> MAPRNEIEETLVTIWQDVLGIEKIGIKDNFYALGGDSIKAIQVAARLHSYQLKLETKDLLKYPTIDQLVHYIKDSKRRSEQGIVEGEIGLTPIQHWFFEQQFTNMHHWNQSYMLYRPNGFDKEILLRVFNKIVEHHDALRMIYKHHNGKIVQINRGLEGTLFDFYTFDLTANDNEQQVICEESARLQNSINLEVGPLVKIALFHTQNGDHLFMAIHHLVVDGISWRILFEDLATAYEQAMHQQTIALPEKTDSFKDWSIELEKYANSELFLEEAEYWHHLNYYT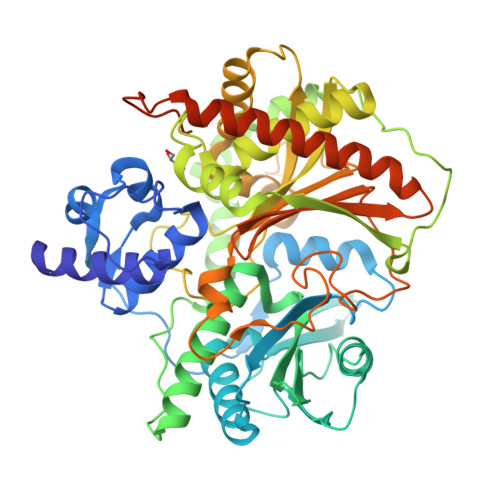DNVQIKKDYVTMNNKQKNIRYVGMELTIEETEKLLKNVNKAYRTEINDILLTALGFALKEWADIDKIVINLEGHGREEILEQMNIARTVGWFTSQYPVVLDMQKSDDLSYQIKLMKENLRRIPNKGIGYEIFKYLTTEYLRPVLPFTLKPEINFNYLGQFDTDVKTELFTRSPYSMGNSLGPDGKNNLGPEGESYFVLNINGFIEEGKLHITFSYNEQQYKEDTIQQLSRSYKQHLLAIIEHCVQKEDTELTPSDFSFKELELEEMDDIFDLLADSLTDDDDKHHHHHH[(2~{R})-1-oxidanylidene-4-phenyl-1-pyrrolidin-1-yl-butan-2-yl]azanium 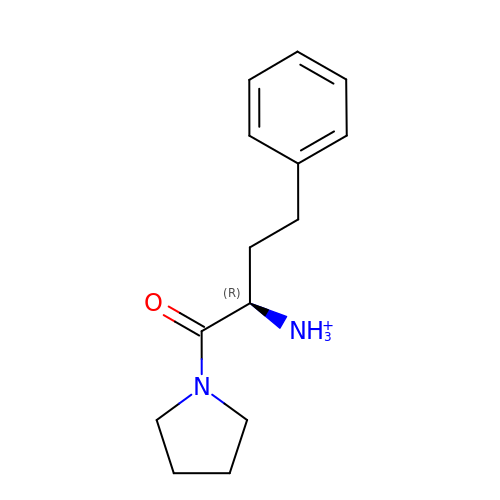| C14 H21 N2 O | WCADMWMQCHZJOA-CYBMUJFWSA-O> 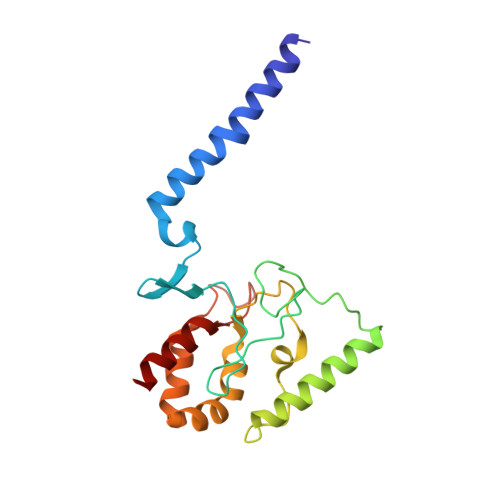LRPALSTFIFLLLITGGVYPLLTTVLGQWWFPWQANGSLIREGDTVRGSALIGQNFTGNGYFHGRPSATAEMPYNPQASGGSNLAVSNPELDKLIAARVAALRAANPDASASVPVELVTASASGLDNNITPQAAAWQIPRVAKARNLSVEQLTQLIAKYSQQPLVKYIGQPVVNIVELNLALDKLDE3,5-bis(3-acetamidophenyl)benzoic acid 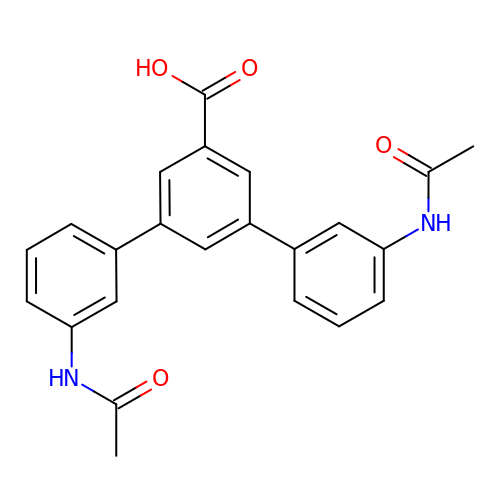| C23 H20 N2 O4 | LLQUGHILDVUZIW-UHFFFAOYSA-N>SQGASVLFGAPGAGDIEVFTTRPDTLFGATYMVLAPEHPLVDQLAADVWPQDTDPRWTGGQDSPRAAIEQYRRSIAAKSDLERQENKEKTGVFTGAYATNPVSGKPVPVFIADYVLLGYGTGAIMAVPGHDQRDWDFANTFGLPVQEVISGGDVT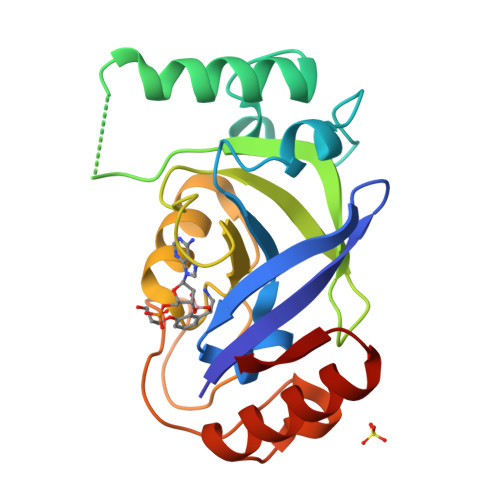KAAYTGDGVLVNSDYLDGLDIEAAKVEVTRRLVKDGRGESR[2x]>TAKSEVEDSKLSIISWNVDGLDTLNLADRARGLCSYLALYTPDVVFLQELIPAYVQYLKKRAVSYLFFEGSDDGYFTGIMLRKSRVKFLESEIICFPTTQMMRNLLIAQVTFSGQKLYLMTSHLESCKNQSQERTKQLRVVLQKIKEAPEDAIVIFAGDTNLRDAEVANVGGLPAGVCDVWEQLGKQEHCRYTWDTKANSNKTVPYVS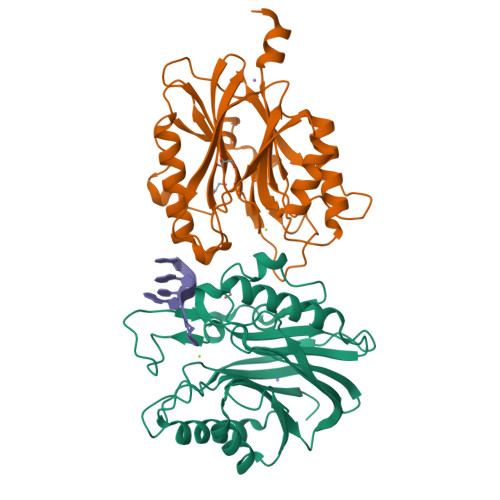RCRFDRIFLRSAKTAPPVTPDHMALIGMEKLDCGRYTSDHWGIYCTFNT[2x]>MTQQIGVIGLAVMGKNLAWNIESRGYSVSVFNRSSEKTDLMVEESKGKNIHPTYSLEEFVNSLEKPRKILLMVQAGKATDATIDSLLPLLDDGDILIDGGNTNYQDTIRRNKALAQSAINFIGMGVSGGEIGALTGPSLMPGGQEEAYNKVADILDAIAAKAKDGASCVTYIGPNGAGHYVKMVHNGIEYADMQLIAESYAMMKELLGMSHEDIAQTFKDWNAGELESYLIEITGDIFMKLDENKEALVEKILDTAGQKGTGKWTSINALELGIPLTIITESVFARFIS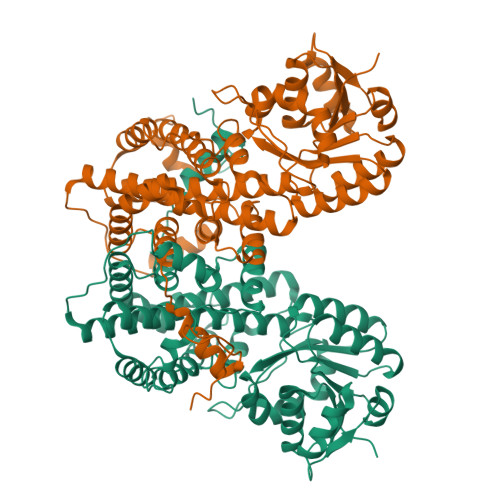SIKEERVNASKELNGPKASFDGDKKDFLEKIRKALYMSKICSYAQGFAQMRKASEDNEWNLKLGDLAMIWREGCIIRAQFLQKIKDAYDNNPGLQNLLLDPYFKNIVTEYQDALRDVVATGVQNGVPTPGFSSSINYYDSYRAADLPANLIQAQRDYFGAHTYERKDKEGVFHTQWIEE[4x]>GGGGTTTTGGGG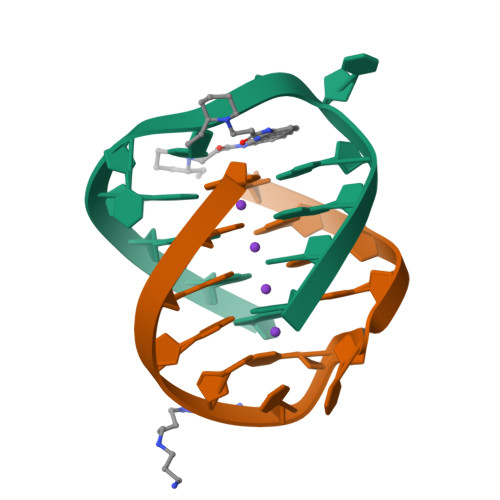[4x]> GPEEEFGMSLIKHNSCVITTENGKFTGLGVYDRFVVVPTHADPGKEIQVDGITTKVIDSYDLYNKNGIKLEITVLKLDRNEKFRDIRRYIPNNEDDYPNCNLALLANQPEPTIINVGDVVSYGNILLS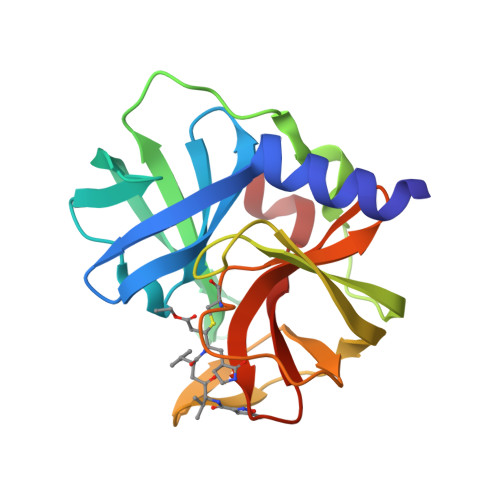GNQTARMLKYSYPTKSGYCGGVLYKIGQVLGIHVGGNGRDGFSAMLLRSYFT>[2x]GPGSMERTFIMIKPDAIKRRLISRIIQRFEEKGLYLAASKCV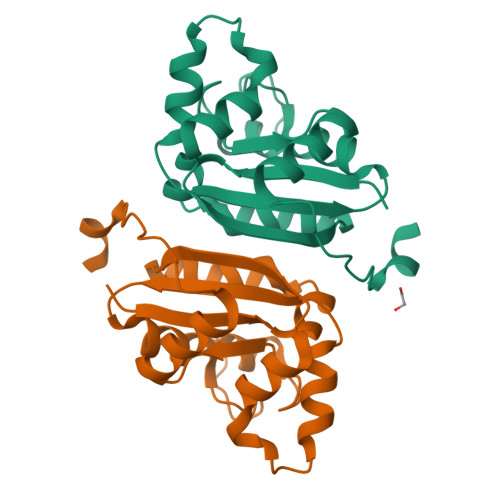IPKREVLETHYSHLSSMPFFSEMVEDMMSGMVLAMVWVGKDAVSIGRKLIGETNPQAASVGTIRGDYGVSTGKNIIHGSDCVENAEKEIKLWIGDDVQPVSFFDKEWIY>[4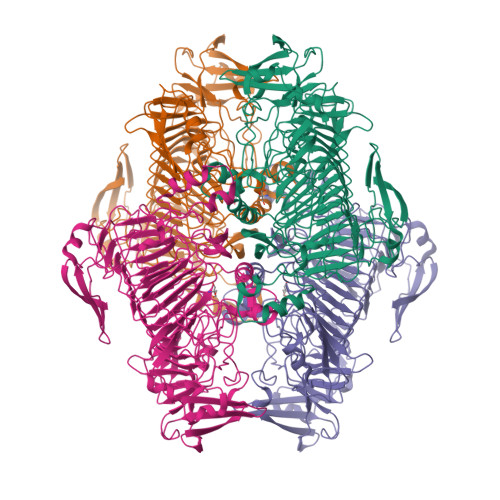x]MEYHVAKTGSDEGKGTLKDPFLTINKAASVAMAGDTIIVHEGVYREWVKPKYKGLSDKRRITYKAAEGEKVVIKGSERIQSWQRVEGNVWRCQLPNSFFGEFNPYKEEVFGDWLLTVNEKKHLGDVYLNGMSFYEVTNYEDLFNPQLRTEVLDHWTQKIVPIKNAEQTKYVWYAEVDREKTTIYANFQGADPNEEFVEINVRRSCFYPVETGIDYITVKGFEMAHAATPWAPPTADQPGLIGPNWSKGWIIEDNIIHDAKCSAISIGKEATTGNNYRSIRKDKPGYQYQLEAVFNAKRNGWSKEKIGSHIIRNNTIYDCGQNAIVGHLGGVFSEIYNNHIYNIALKREFYGHEIAGIKLHAAIDVQIHHNRIHDCSLGLWLDWEAQGTRVSKNLFYNNNRDVFVEVSHGPYLVDHNILSSEYAIDNMSQGGAYINNLIAGKMNQRKVLNRSTQYHLPHSTEVAGFAFVYGGDDRFYNNIFIGKEGLENVGTSHYNNCTTSLEEYIEKVNEVPGDLGEFERVEQPVYINKNAYFNGAEPFEKEKDNLVKKDFDPKLAIIDEGDEVYLSLQLPDEFENIVGDIHSTKTLERVRIVDAEYESPDGKELVLDTDYLDAKKPENSSIGPIALLKKGNNYIKVW Using multidisciplinary approaches, we showed that two long coiled-coil proteins, Cep63 and Cep152, form a heterotetrameric building block that undergoes a stepwise formation into higher molecular weight complexes, ultimately generating a cylindrical architecture around a centriole. Remarkably, Cep63 and Cep152 can self-assemble into a radially aligned, submicrometer-scale, cylindrical structure in vitro in such a fashion that the N-termini of Cep63 and Cep152 are placed at the innermost and outermost regions, respectively, of the structure. Notably, the N-terminus of Cep63 (i.e., the mCherry fluorescence of Cep63) was detected in the innermost region (231 ± 23 nm in diameter), whereas the N-terminus of Cep152 (i.e., the mGFP fluorescence of Cep152) was positioned at the outermost region (350 ± 23 nm in diameter). These observations agree with the previously proposed model that Cep63 and Cep152 generate an antiparallel 2:2 heterotetrameric complex arranged around a centriole in the Cep152 N-terminus-outward fashion. Mutants defective in Cep63•Cep152 heterotetramer formation displayed crippled pericentriolar Cep152 organization, polo-like kinase 4 (Plk4) relocalization to the procentriole assembly site, and Plk4-mediated centriole duplication.

Comparative analysis of the Cep63 (462–483) region with the previously characterized GCN4 leucine-zipper dimer38 revealed their structural similarity, each showing pairwise hydrophobic interactions along its parallelly arranged dimer (right). Notably, three copies of the Cep63 (440–490) dimer were found in an asymmetric unit (left) within which two copies appeared to be from crystal-packing artifacts, judging from several lines of evidence. First, the data obtained from SAXS, sedimentation velocity/equilibrium, and iSCAMS analyses are all consistent with the dimeric form of Cep63 (440–541). Second, SEC-multi-angle light scattering (MALS) showed that Cep63 (440–490) is mainly (97.9%) in a dimeric state. Third, the L469A N473R V480K mutations designed to disrupt the parallelly arranged dimeric interactions yielded a delayed peak (12.82 mL) of the monomeric form, whereas the L445A A456K L463K mutations aimed at disrupting the predicted packing interactions did not. Fourth, the Cep63 N-terminus-in and C-terminus-out arrangement observed around a centriole does not support a tridirectional protein orientation that a hexameric Cep63 could adopt (left). Intriguingly, the Cep63 (440–490) fragment is highly acidic (pI approximately 5.5), raising the possibility that the open-ended N-termini of the Cep63 (440–490) dimer could interact with the conserved basic Cep152 (1273–1295) region (pI of 9.5) predicted to form a CC motif. If this were the case, then the Cep152 (1273–1295) region could substitute the packing interface observed in the Cep63 (440–490) crystal structure.

>[12x]GSEFMDMEKRLRAEMQKAEDKAVEHKEILDQLESLKLENRHLSEMVMKLELGLHEA> AVNGKGMNPDYKAYLMAPLKKIPEVTNWETFENDLRWAKQNGFYAITVDFWWGDMEKNGDQQFDFSYAQRFAQSVKNAGMKMIPIISTHQCGGNVGDDCNVPIPSWVWNQKSDDSLYFKSETGTVNKETLNPLASDVIRKEYGELYTAFAAAMKPYKDVIAKIFLSGGPAGELRYPSYTTSDGTGYPSRGKFQAYTEFAKSKFRLWVLNKYGSLNEVNKAWGTKLISELAILPPSDGEQFLMNGYLSMYGKDYLEWYQGILEN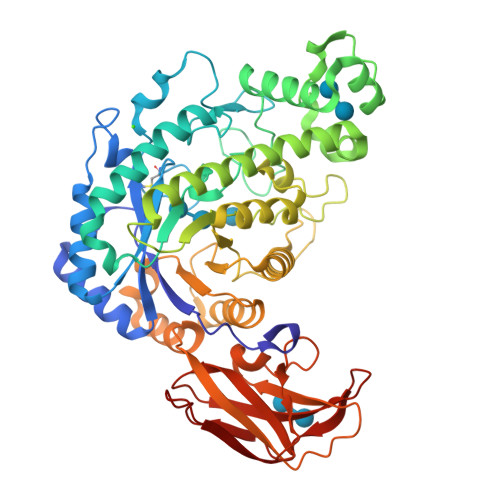HTKLIGELAHNAFDTTFQVPIGAKIAGVHWQYNNPTIPHGAEKPAGYNDYSHLLDAFKSAKLDVTFTCLEMTDKGSYPEYSMPKTLVQNIATLANEKGIVLNGENALSIGNEEEYKRVAEMAFNYNFAGFTLLRYQDVMYNNSLMGKFKDLLGVTPVMQTIVVKNVPTTIGDTVYITGNRAELGSWDTKQYPIQLYYDSHSNDWRGNVVLPAERNIEFKAFIKSKDGTVKSWQTIQQSWNPVPLKTTSHTSSW> MKDQLSDEQKETILKALNDAIEKGPWDKSNFLRVIGKKLIAIRDRFLKRIGAASQAK;> EIGEP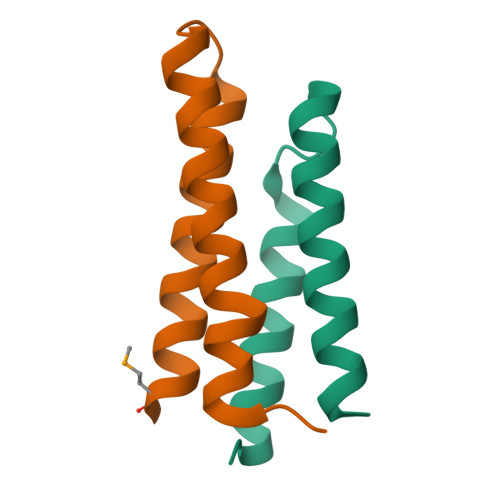DVTDATLGSVYSEIISPVKDCILTVAKAVSFNPGGKDNTDAVEVLTELNTKVERAAMNQPILTTKTER>[5x]MAELPPGRLATTEDYFAQQAKQAVTPDVMAQLAYMNYIDFISPFYSRGCSFEAWELKHTPQRVIKYSIAFYAYGLASVALIDPKLRALAGHDLDIAVSKMKCKRVWGDWEEDGFGTDPIEKENIMYKGHLNLMYGLYQLVTGSRRYEAEH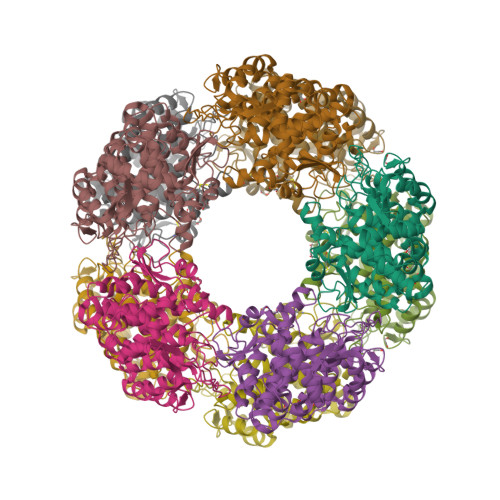AHLTRIIHDEIAANPFAGIVCEPDNYFVQCNSVAYLSLWVYDRLHGTDYRAATRAWLDFIQKDLIDPERGAFYLSYHPESGAVKPWISAYTTAWTLAMVHGMDPAFSERYYPRFKQTFVEVYDEGRKARVRETAGTDDADGGVGLASAFTLLLAREMGDQQLFDQLLNHLEPPAKPSIVSASLRYEHPGSLLFDELLFLAKVHAGFGALLRMPPPAAKLAGK> VTGTNKVGTGKGVLGDTKSLNTTLSGSSYYLQDNTRGATIFTYDAKNRSTLPGTLWADADNVFNAAYDAAAVDAHYYAGKTYDYYKATFNRNSINDAGAPLKSTVHYGSNYNNAFWNGSQMVYGDGDGVTFTSLSGGIDVIGHELTHAVTENSSN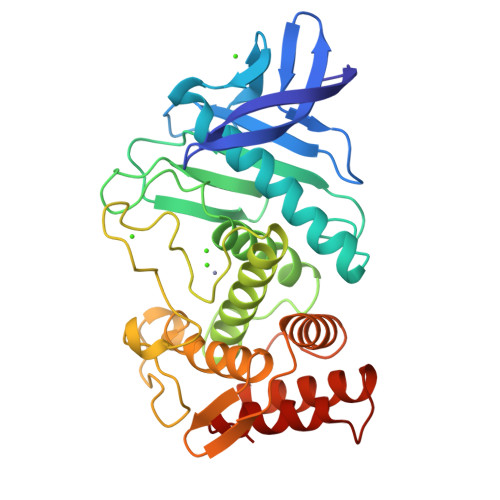LIYQNESGALNEAISDIFGTLVEFYDNRNPDWEIGEDIYTPGKAGDALRSMSDPTKYGDPDHYSKRYTGSSDNGGVHTNSGIINKQAYLLANGGTHYGVTVTGIGKDKLGAIYYRANTQYFTQSTTFSQARAGAVQAAADLYGANSAEVAAVKQSFSAVGVN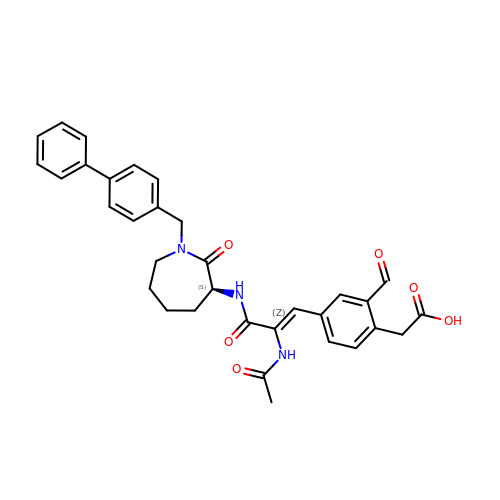[4-((1Z)-2-(ACETYLAMINO)-3-{[1-(1,1'-BIPHENYL-4-YLMETHYL)-2-OXOAZEPAN-3-YL]AMINO}-3-OXOPROP-1-ENYL)-2-FORMYLPHENYL]ACETIC ACID | C33 H33 N3 O6 | NKMPOVPTYDXGEC-MNRBYUMSSA-N Recently, a shortened Dscam (sDscam) gene family with tandemly arrayed 5′ cassettes in Chelicerata species has been identified, which encodes ∼50–100 isoforms. Chelicerata sDscams could be classified into two subfamilies, sDscamα and sDscamβ, containing one and two variable Ig domains, respectively. Crystal structures and cell aggregation assays demonstrated that both α and β subfamilies of sDscam used Ig1 for the isoform-specific trans recognition in a hand-in-hand manner. Furthermore, the cis interactions were established by the three FNIII domains of sDscam, which assemble into a cross fold with a kink between FNIII2 and FNIII3.

We found that FNIII2 alone but not FNIII1 or FNIII3 could promote cKIT tyrosine phosphorylation, suggesting the essential role of FNIII2 domain in mediating sDscam cis interactions. The gel-filtration analysis supported our observations in the crystal structures: Ig1 mediated the formation of trans homodimer and all the three FNIII domains were involved in the cis interactions.

> GASAPIGAPTDVNVEPIGSRTLKVTWRPPLVDHWNGIIKGYYVGHKESDSSQQYRYQRVERSGINPETLLIAGLQKAKVYNVVVKAFNTAGSGPESHPVEAYSLE>[4x]GSHMGTVRQTSGPALARGDKVAVVSIANYTETPDAGHS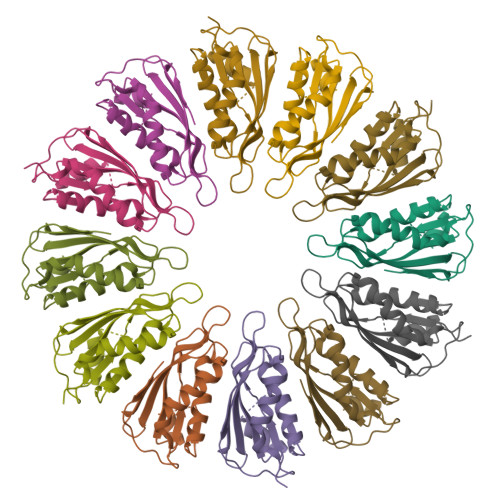AESIAANTLRAGGIADVRIAPADSNRNSLFDTTQRADSDKALEWARSQNARYVLSGAVEEWRYKTGVDGEPVVGVTFELIDVSNGAVVWSATGTRTGWSRSGLSSVATSLIAKVLSPLQARQ>MEAVLNELVSVEDLLKFEKKF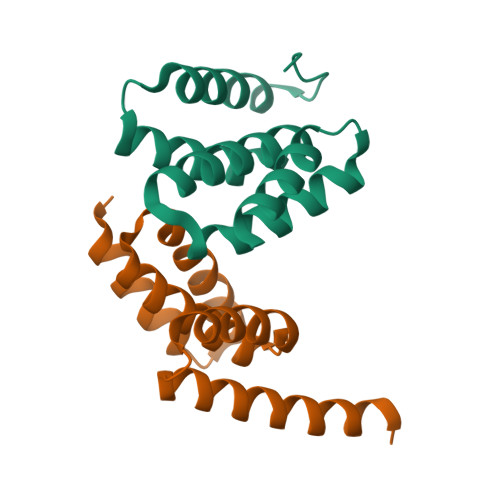QSEKAAGSVSKSTQFEEAWCLVRSKYNDDIRKGIVLLEELLPKGSKEEQRDYVFYLAVGNYRLKEYEKALKYVRGLLQTEPQNNQAKELERLIDKAMKKDGLLEVLFQ[2x]> ADLTSHHHHHHVEPARITLTYKEGAPITIMDNGNIDTELLVGTLTLGGYKTGTTSTSVNFTDAAGDPM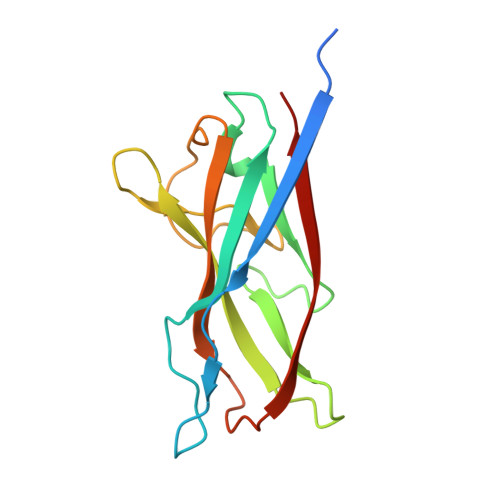YLTFTSQDGNNHQFTTKVIGKDSRDFDISPKVNGENLVGDDVVLATGSQDFFVRSIGSKGGKLAAGKYTDAVTVTVSNQ>[2x]MLPGTFFEVLKNEGVVAIAT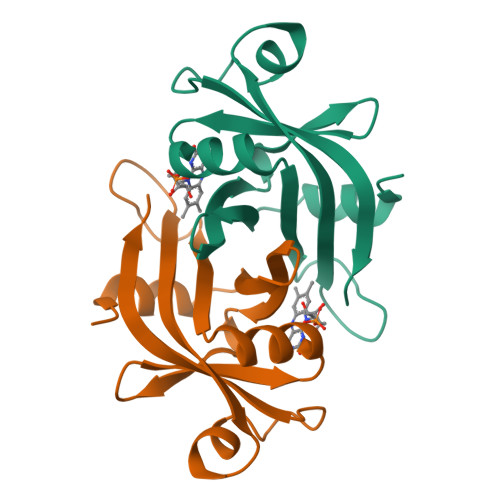QGEDGPHLVNTWNSYLKVLDGNRIVVPVGGMHKTEANVARDERVLMTLGSRKVAGRNGPGTGFLIRGSAAFRTDGPEFEAIARFKWARAALVITVVSAEQTK>[2x]MFLKKLIEAKKAYTFDDVLLVPNASWVEPKDTDVSTDLAGLKLNIPIVSAAMDTVTEKEMAIALARLGGLGVIHRNMSIEEQVHQVQAVKKADEVVIGSGGYPQAARDKKGRLLVAAACGPHDFERAKALIEAEVDAIAIDCAHAHNMRVVENV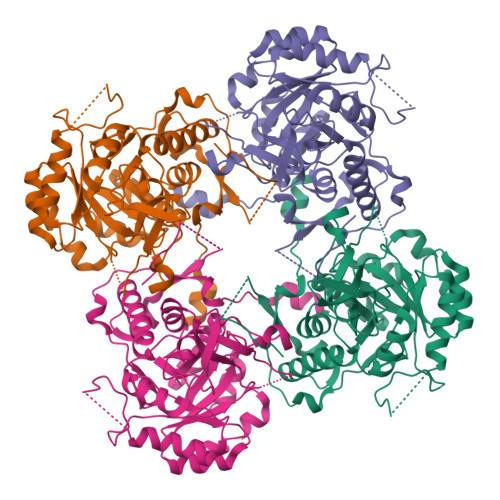KKFKEMLEGTDIKLIVGNIATKEAAEDLIKAGADVLKVGIGPGSICTTRVVAGVGVPQLTAVAEVADVAKEHNVPIIADGGIRYSGDIAKAIAAGADAVMLGSLLAGTDEAPGQLMVINGRKYKQYRGMGSLGAMTGGVGAGADRYFQAPAKSHMKHVKLVPEGVEGAVPYKGPVSEVVFQLIGGLRASMGYCGAKNLKEMQEKARFVIITPSGQVESHPHDIIITNEAPNYPLGKLEHHHHHH In the 3′ to 5′ pathway, the mRNA body is processively hydrolyzed by the 10-component cytoplasmic exosome complex (exo-10; exo-9 plus Rrp44/Dis3), followed by the removal of the cap structure of the remaining short RNA fragment by the Scavenger Decapping enzyme DcpS (Dcs1p in yeast). The apo DcpS decapping enzyme assembles into an 80-kDa symmetric homodimer that contains dimeric N- and C-terminal domains that are linked by a flexible hinge region. The enzyme possesses two bipartite active sites that are located at the interface between the N- and C-terminal domains. Upon substrate binding to the C-terminal part of one of the active sites, the N-terminal domain flips over to enclose the mRNA substrate in a well-defined pocket.

Next, we aimed at determining whether this preference in substrate usage is a conserved mechanism, and we focused on the enzymes from Chaetomium thermophilum (a thermophilic filamentous fungus) and humans. The protein crystallized in space group P1 with one dimer per asymmetric unit. The structure was determined by molecular replacement and refined to a resolution of 1.95 Å with good geometry. DcpS forms a symmetric dimer with the same overall fold as the human and mouse protein, indicating that the fold and domain orientation of the protein is conserved despite a relatively low sequence conservation. The C. thermophilum and human apo proteins show a single set of peaks (black contours), which confirms the findings from static crystal structures. Upon addition of an mRNA substrate with one nucleotide (red contours), the C. thermophilum and human enzymes undergo a transition into an asymmetric conformation, thereby forming a catalytically competent active site. On the contrary, an mRNA substrate of three nucleotides does not result in the formation of the closed conformation (blue contours). From these data, we conclude that the length sensing mechanism that we identified in the S. cerevisiae protein is conserved in the C. thermophilum and human enzymes.

>GAMDAKRSAEALVPRFQFERLLNQDQAGRRSALYGAIDGQPALLILERAPFPTSTAYLGRAANTLRALTNLGANDIYHWYLASSGVIEIPVEESEGTDDEFADLKINLIYPCTEKHVKKYSKQGVRFVTETPEIYRDYVRPYMQAQREAGRLNWVYNIIEGRKEVEDVIYRTPYGQDPEEGFLLLPDLNWDRKTVEALHLLGIVERRDLWSLRDLKKKHLPWLRHMREKLIEATTKVYPTVEADQLKLYLHYQPTYYHLNIHIVHVQLEAGATQATGKAVGLESVMEQLEHMHVGPEDGDGSDVGMDRVTMCYTLGEASDLWVDVFEPLKRKKQARPTSEPGAASQSQ[2x]>CSAMGTAIKK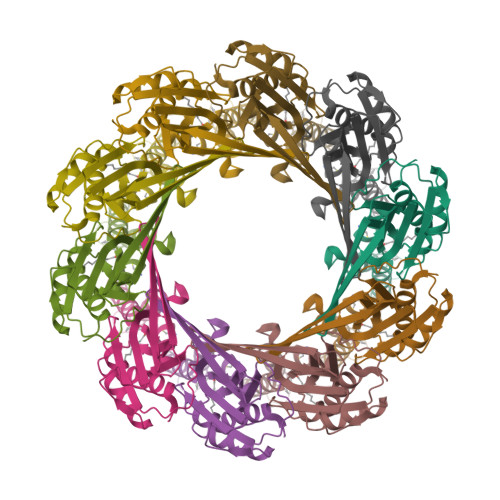RNLEVKTQMSETIWLEPSNNKTVYLQIKNTSDKDMSGLQAKIASAVTSKGYQVVSNPDTAGYWIQANVLKADKMDLRESQGWLSRGYEGAVTGAALGAGITAYNSSSAGATLGVGLAAGLVGMAADAMVEDVNYTMITDVQIAERTKTQVQTDNVAVLRQGTSGTKVQTSTETGNQHKYQTRVVSNANKVNLKFPEAQPVLEDQLAKSIANILGSG[10x]> EW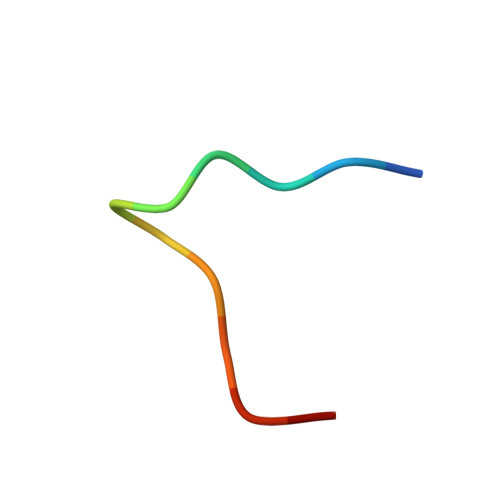VHPQFEQKAK> GYDEIEELKSKNEVLTNLLNKLIAFDKKRIFLYPVNVQLVPDYLNVIKEPMDFTTMKQKLQNFKYKSFQEFEKDVLLIINNCYTYND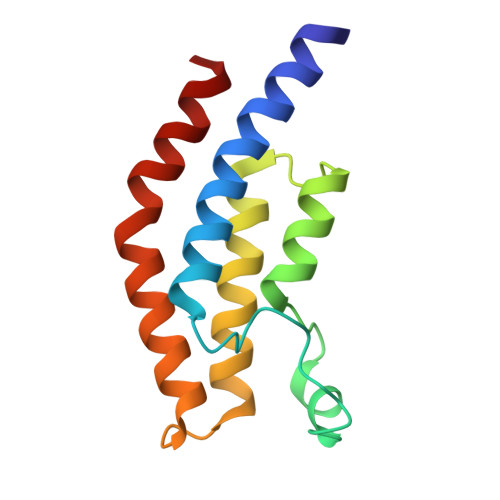PSTIYYKFAEDIETYYKKLNIKIQTKYMNIHL> ADDIVLKAKNGDVKFPHKAHQKAVPDCKKCHEKGPGKIEGFGKE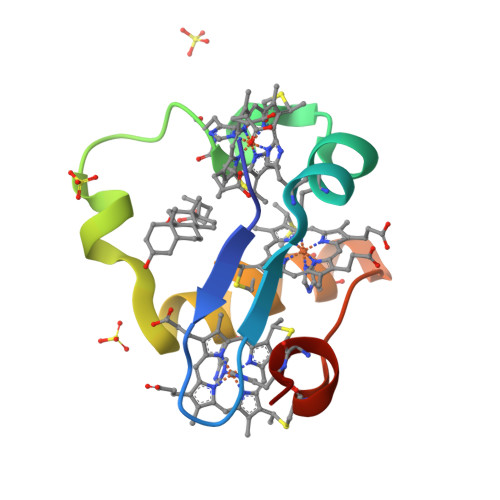MAHGKGCKGCHEENKKGPTKCGECHKK> GSPDPRAELDSTVLLTRSLLADTRQLAAQLRDKFPADGDHNLDSLPTLAMSAGALGALQLPGVLTRLRADLLSYLRHVQWLRRAGGSSLKTLEPELGTLQARLDRLLRRLQLLMSRLALPQPPPD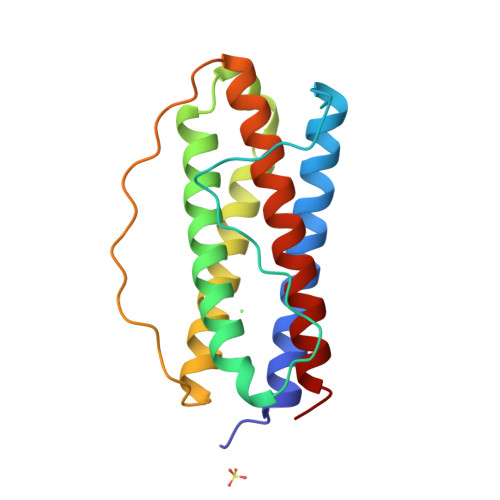PPAPPLAPPSSAWGGIRAAHAILGGLHLTLDWAVRGLLLLKTRL> AHHHHHHTSGDDDDKAKKKLPKCQKQEDCGSWDLKCNNVTKKCECRNQVCGRGCPKERYQRDKYGCRKCLCKGCDGFKCRLGCTYGFKTDKKGCEAFCTCNTKETACVNIWCTDPYKCNPESGRCED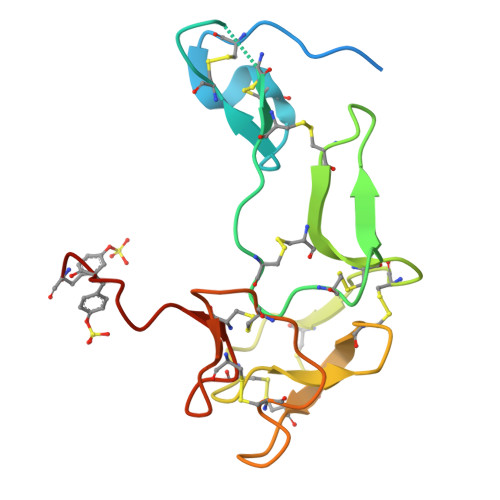PNEEYEYDYE>MPAGHEEFDIPFPSRVNPFHARAEDRHVAWMRAMGLITGDAAEATYRRWSPAKVGARWFYLAQGEDLDLGCDIFGWFFAYDDHFDGPTGTDPRQTAAFVNRTVAMLDPRADPTGEHPLNIAFHDLWQRESAPMSPLWQRRAVDHWTQYLTAHITEATNRTRHTSPTIADYLELRHRTGFMPPLLDLIERVWRAEIPAPVYTTPEVQTLLHTTNQNINIVNDVLSLEKEEAHGDPHNLVLVIQHERQSTRQQALATARRMIDEWTDTFIRTEPRLPALCGRLGIPLADRTSLYTAVEGMRAAIRGNYDWCA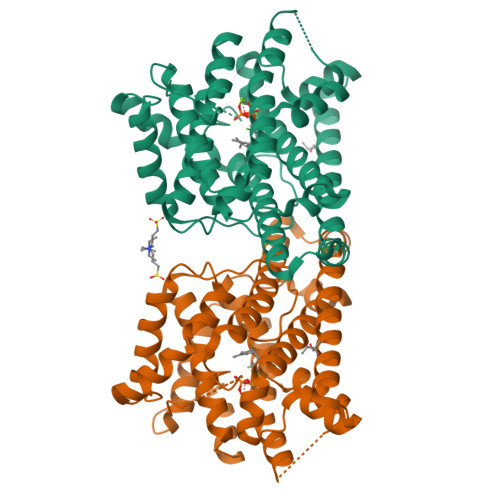ETNRYAVHRPTGTGRATTPW[2x]> UAG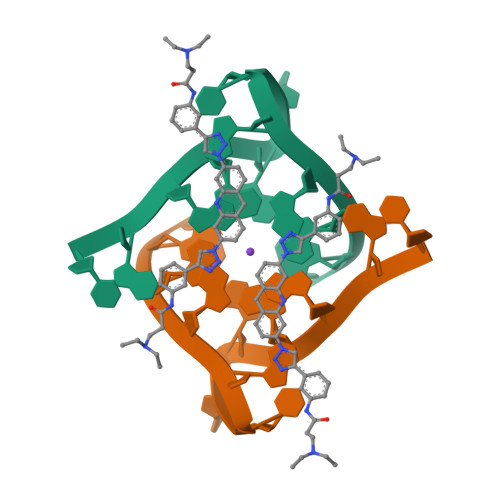GGUUAGGGU> MSSNTDIIALLSSDADKAVDQIIEDSKRLHIVVNGTGTEQAVAEDGSLLPSVRKALIDNLYFKTPPLPWRNGGSVNEFNQLYSFTDVSGNTTWWYAPGATVSNPVVMRDSPINDGKFKVFLDKTNIADIYAPLNSPNFVGNPRVPTPAPGDNSQSIPT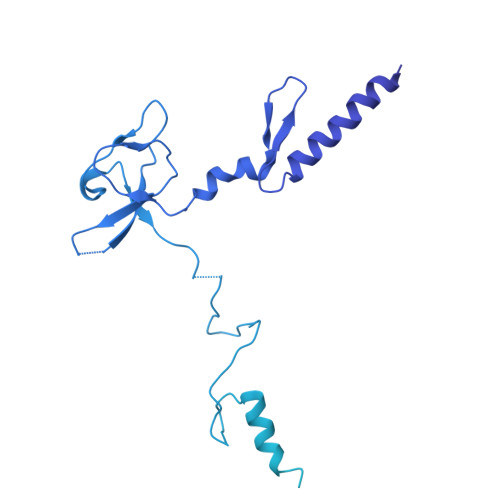TGWVQSEMEGLEDLIISSMRGEFENITVRNDAILQDTYINGEFIVTSDKLAAANTEATFRRIRMVGTGTTGTAATEIAFEQNTTPPPGVSTKTNIKPFAVSTGILTVDQINGKAAQVGDVAVSTDSLNVDGYMRGDYLHLEGNNRNTAGRPQLIVDGIAEIETLRVTGTIEGVKADVDGLDIHPRSVIVDEGLTVAKDTTMTGKLTVGGTTKVGNLEVTGTLSGVAISVDGKDIKPRSVNTGNLVATGDVQISGTTTATGKITTQDLEVLGTLTANLDLSGSDLSVDNINVAQTATITDLVVTGTTTGVKGDVEGEAIAPASVAATGTVSAASMSTTGNMAVGGNLTITGDFRPASVAGQDTPRLVVQGDSDLQGDLNVSGTITGVVDLTAQDINMNSLGLAQGLTAGGGITSFSTVKGVNGVFGEGSTAPGAIGLQSMTNAKVATDLLVGEDLRVEGDTNLFGNLSVTGTITGNMNFSGKTIAPATVNATTVTATNLTVTGTIDLTDSPIVAQEITATNVEATGKMVAGKYSTTPKTANATTATFTPDGTTSIYNVNVQADTEVQAPAGLLSSGKGESIFIYFEQDTTGHAVTFSSAFVVHNAATVSNAANSITIANLVYRGTGPLIDVFLTGR>[12x]SNAMGENVLICLCGSVNSINISHYIIELKSKFDEVNVIASTNGRKFINGEILKQFCDNYYDEFEDPFLNHVDIANKHDKIIILPATSNTINKIANGICDNLLLTICH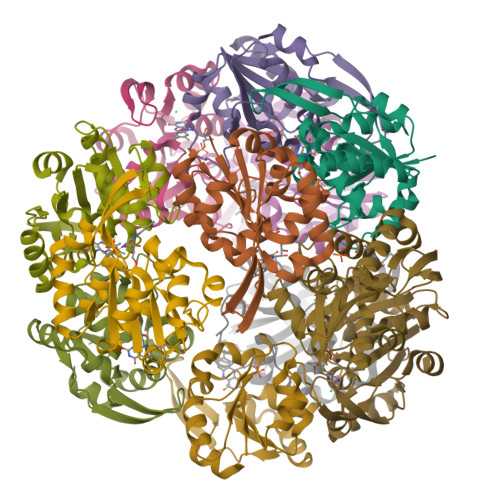TAFEKLSIFPNMNLRMWENPVTQNNIRLLKDYGVSIYPANISESYELASKTFKKNVVAPEPYKVLEFI>QLTFQTSSPAHLTMPYVMPGDGEVVGVGEPVAIRFDENIADRGAAEKAIKITTNPPVEGAFYWLNNREVRWRPEHFWKPGTAVDVAVNTYGVDLGEGMFGEDNVQTHFTIG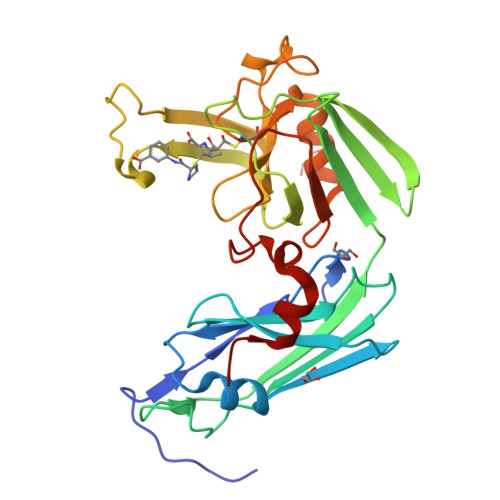DEVIATADDNTKILTVRVNGEVVKSMPTSMGKDSTPTANGIYIVGSRYKHIIMDSSTYGVPVNSPNGYRTDVDWATQISYSGVFVHSAPWSVGAQGHTNTSHGCLNVSPSNAQWFYDHVKRGDIVEVVNTVGGTLPGIDGLGDWNIPWDQWRAGNAKA[2x]>DVLRDLMDLKSNADSGDVSAQFELSRRYLNGDGLEQNDDEAIRWLRMAAEGGLPRAQAGLGWMYAAGRGVNKDETLSFSWYERAAVAGFPVAQYMLGRYYEKGIGVAKDRVLAKEWYEKAAAQGNEKA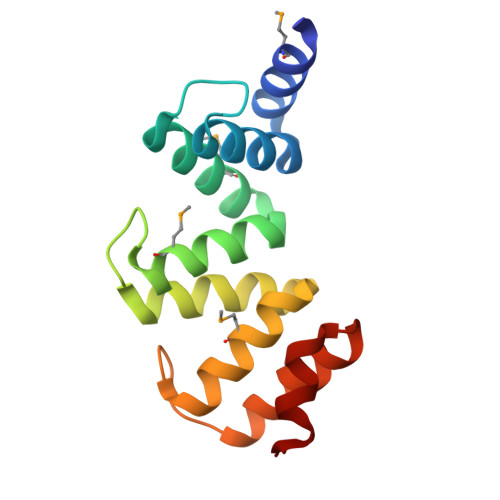KKRLQDW[2x]>[2x]MAFYSCCWVLLALTWHTSAYGPDQRAQKKGDIILGGLFPIHFGVAAKDQDLKSRPESVECIRYNFRGFRWLQAMIFAIEEINSSPALLPNLTLGYRIFDTCNTVSKALEATLSFVAQNKIDSLNLDEFCNCSEHIPSTIAVVGATGSGVSTAVANLLGLFYIPQVSYASSSRLLSNKNQFKSFLRT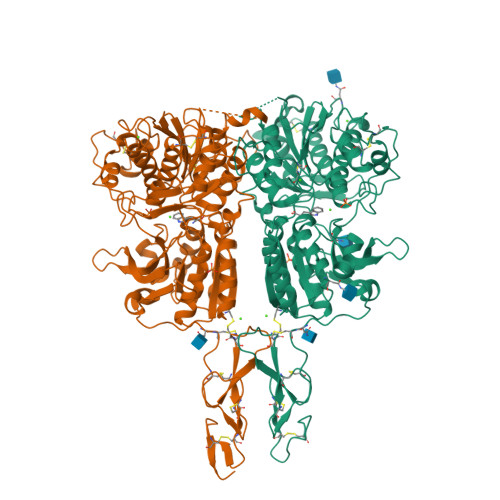IPNDEHQATAMADIIEYFRWNWVGTIAADDDYGRPGIEKFREEAEERDICIDFSELISQYSDEEEIQHVVEVIQNSTAKVIVVFSSGPDLEPLIKEIVRRNITGKIWLASEAWASSSLIAMPQYFHVVGGTIGFALKAGQIPGFREFLKKVHPRKSVHNGFAKEFWEETFNCHLQEGAKGPLPVDTFLRGHEESGDRFSQSSTAFRPLCTGDENINSVETPYIDYTHLRISYNVYLAVYSIAHALQDIYTCLPGRGLFTNGSCADIKKVEAWQVLKHLRHLQFTNNMGEQVTFDECGDLVGNYSIINWHLSPEDGSIVFKEVGYYNVYAKKGERLFINEEKILWSGFSREVPFSNCSRDCLAGTRKGIIEGEPTCCFECVECPDGEYSDETDASACNKCPDDFWSNENHTSCIAKEIEFLSDYKDDDDK> MAFSVNYDSSFGGYSIHDYLGQWASTFGDVNHTNGNVTDANSGGFYGGSLSGSQYAISSTANQVTAFVAGGNLTYTLFNEPAATLY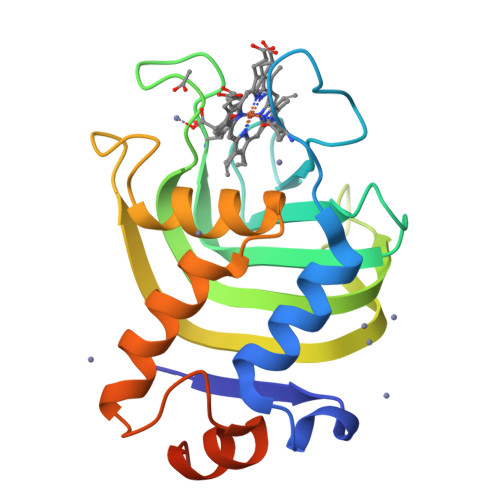GQLDSLSFGDGLSGGDTSPYSIQVPDVSFGGLNLSSLQAQGHDGVVHQVVYGLMSGDTGALETALNGILDDYGLSVNSTFDQVAAATAVGVQHADSPELLAA>HHHHHSSGLVPRGSHMTNPAYFPQLSQLDVSGEMESTYEDIRLTLRVPWVAFGCRVLATFPGYLPLAWRRSAEA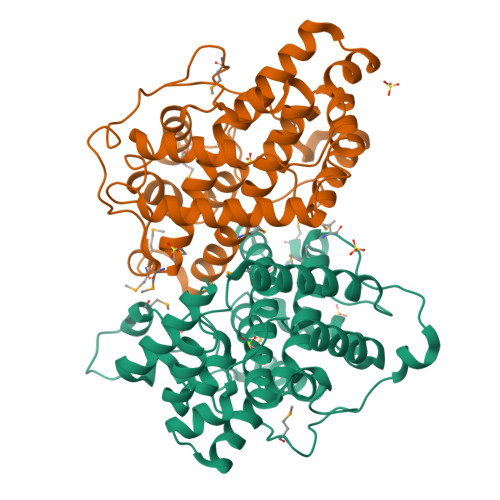LITRYAEQAADELRERSLLNIGPLPNLKERLYAAGFDDGEIEKVRRVLYAFNYGNPKYLLLITALSESMQMRPVGGAEVSSELRASIPKGHPKGMDPLLPLVDATKASTEVQGLLKRVADLHYHHGPASDFQALANWPKVLQIVTDEVLAPVARTEQYDAKSRELVTRARELVRGLPGSAGVQRSELMSMLTPNELAGLTGVLFMYQRFIADITISIIHITECLDGAEAASKSPFPI[4x]> KKSWDEMSCAEKLFKVLSFGLWNPTYSRSERQSFQELLTVLEPVYPLPNELGRVSARFSDGSSLRISVTNSELVEAEIRTANNEKITVLLESNEQNRLLQSLPIDRHMPYIQVHRALSEMDLTDTTSMRNLLGFTSKLSTTLIPHNAQTDPLSGPTPFSSIFMDTCRGLGNAKLSLNGVDIPANAQKLLRDALGLKDTHSSPTRNVIDHGISRHDAEQIARESSGSDKQKAEVVEFLCHP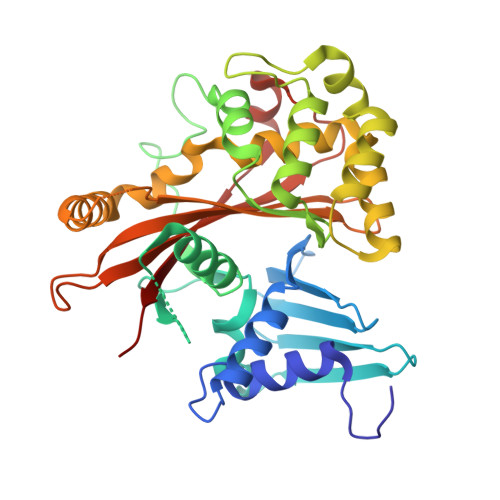EAATAICSAFYQSFNVPALTLTHERISKASEYNAERSLDTPNACINISISQSSDGNIYVTSHTGVLIMAPEDRPNEMGMLTNRTSYEVPQGVKCIIDEMVSALQPRYAASETYLQNT>AMAHHHHHHLVPRGSEASTPGDLVSIPTAISRAEGKITSALGSNQDVVDRIYKQVALESPLALLNTESIIMNAITSLSYQIN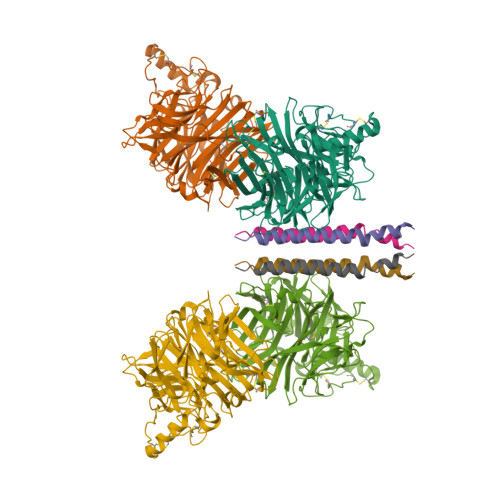GAANNSGCGAPVHDPDYIGGIGKELIVDDTSDVTSFYPSAFQEHLNFIPAPTTGSGCTRIPSFDMSATHCYTHNVIFSGCRDHSHSHQYLALGVLRTSATGRVFFSTLRSINLDDTQNRKSCSVSATPLGCDMLCSKVTETEEEDYNSVIPTSMVHGRLGFDGQYHEKDLDVTTLFGDWVANYPGVGGGSFIDNRVWFPVYGGLKPSSPSDTAQEGRYVIYKRYNDTCPDEQDYQIRMAKSSYKPGRFGGKRVQQAILSIKVSTSLGEDPVLTIPPNTVTLMGAEGRVLTVGTSHFLYQRGSSYFSPALLYPMTVNNNTATLHSPYTFNAFTRPGSVPCQASARCPNSCVTGVYTDPYPLVFHRNHTLRGVFGTMLDDEQARLNLVSAVFDNISRSRITRVSSSRTKAAYTTSTCFKVVKTNKTYCLSIAEISNTLFGEFRIVPLLVEILKDDGV[4x]>TLGNTT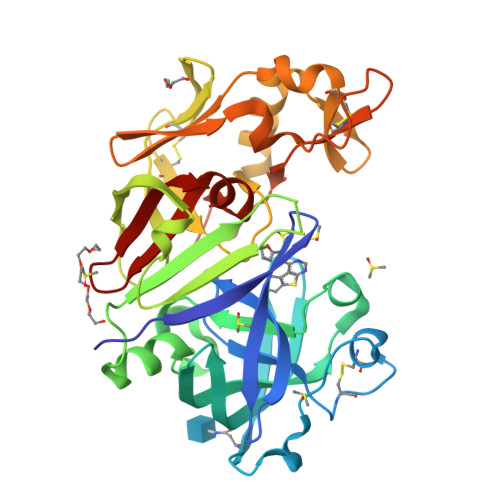SSVILTNYMDTQYYGEIGIGTPPQTFKVVFDTGSSNVWVPSSKCSRLYTACVYHKLFDASDSSSYKHNGTELTLRYSTGTVSGFLSQDIITVGGITVTQMFGEVTEMPALPFMLAEFDGVVGMGFIEQAIGRVTPIFDNIISQGVLKEDVFSFYYNRDSENSQSLGGQIVLGGSDPQHYEGNFHYINLIKTGVWQIQMKGVSVGSSTLLCEDGCLALVDTGASYISGSTSSIEKLMEALGAKKRLFDYVVKCNEGPTLPDISFHLGGKEYTLTSADYVFQESYSSKKLCTLAIHAMDIPPPTGPTWALGATFIRKFYTEFDRRNNRIGFALAR[2x]>GSHMFQCNVPLGMESGRIANEQISASSTYSDGRWTPQQSRLHGDDNGWTPNLDSNKEYLQVDLRFLTMLTAIATQGAIS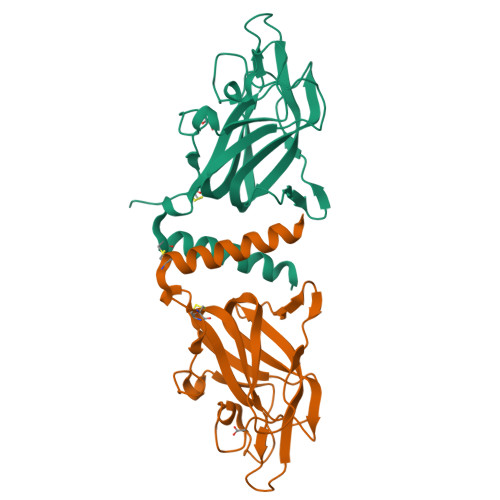RETQNGYYVKSYKLEVSTNGEDWMVYRHGKNHKVFQANNDATEVVLNKLHAPLLTRFVRIRPQTWHSGIALRLELFGCRVTDAPCSNMLGMLSGLIADSQISASSTQE[2x]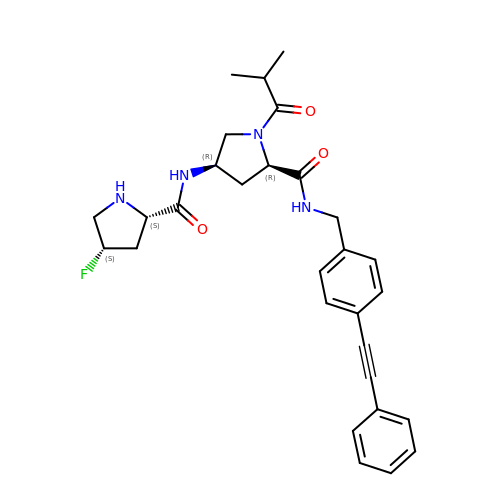(2~{R},4~{R})-4-[[(2~{S},4~{S})-4-fluoranylpyrrolidin-2-yl]carbonylamino]-1-(2-methylpropanoyl)-~{N}-[[4-(2-phenylethynyl)phenyl]methyl]pyrrolidine-2-carboxamide | C29 H33 F N4 O3 | VUQQJEHSKZCJDR-ROXDYWFKSA-N>AATTVNGGTVHFKGEVVNAACAVDAGSVDQTVQLGQVRTASLAQEGATSSAVGFNIQLNDCDTNVASKAAVAFLGTAIDAGHTNVLALQSSAAGSATNVGVQILDRTGAALTLDGATFSSETTLNNGTNTIPFQARYFATGAATPGAANADATFKVQYQ[6x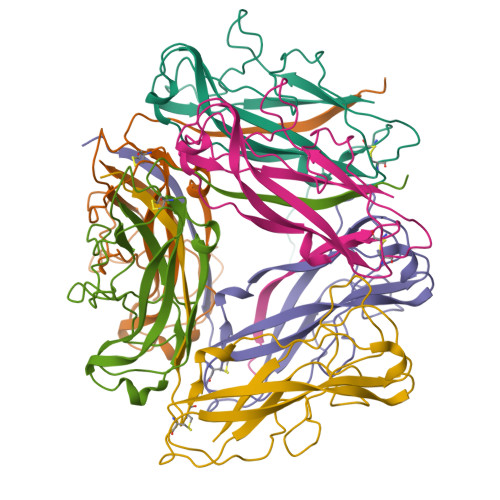]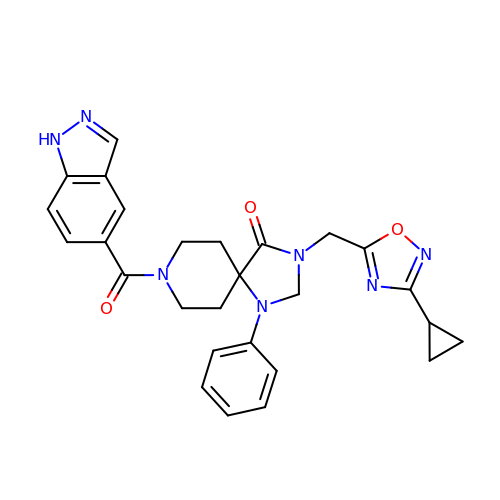3-[(3-cyclopropyl-1,2,4-oxadiazol-5-yl)methyl]-8-(1~{H}-indazol-5-ylcarbonyl)-1-phenyl-1,3,8-triazaspiro[4.5]decan-4-one | C27 H27 N7 O3 | SCNJPRUXBGWNTB-UHFFFAOYSA-N5-methyl-L-tryptophan | C12 H14 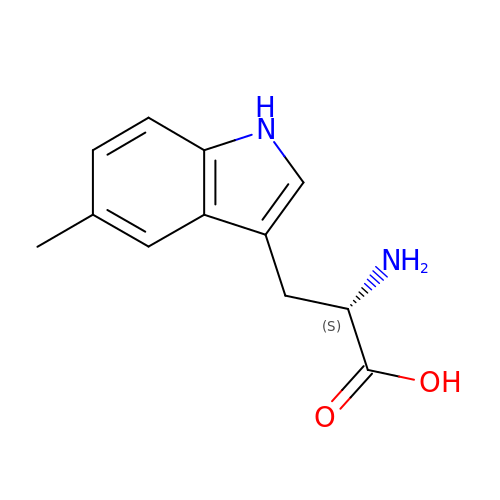N2 O2 | HUNCSWANZMJLPM-JTQLQIEISA-N>[2x]MAH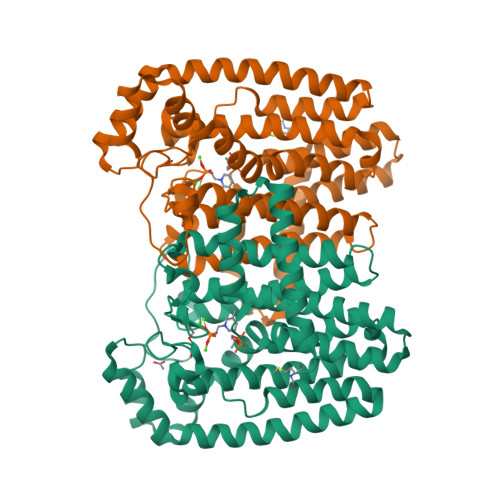MERFQKVYEEVQEFLLGDAEKRFEMDVHRKGYLKSMMDTTCLGGKYNRGLCVVDVAEAMAKDTQMDAAAMERVLHDACVCGWMIEMLQAHFLVEDDIMDHSKTRRGKPCWYLHPGVTAQVAINDGLILLAWATQMALHYFADRPFLAEVLRVFHDVDLTTWIGQLYDVTSMVDSAKLDAKVAHANTTDYVEYTPFNHRRIVVYKTAYYTYWLPLVMGLLVSGTLEKVDKKATHKVAMVMGEYFQVQDDVMDCFTPPEKLGKIGTDIEDAKCSWLAVTFLTTAPAEKVAEFKANYGSTDPAAVAVIKQLYTEQNLLARFEEYEKAVVAEVEQLIAALEAQNAAFAASVKVLWSKTYKRQK> MEEIYAKFVSQKISKTRWRPLPPGSLQTAETFATGSWDNEENYISLWSIGDFGNLDSDGGFEGDHQLLCDIRHHGDVMDLQFFDQERIVAASSTGCV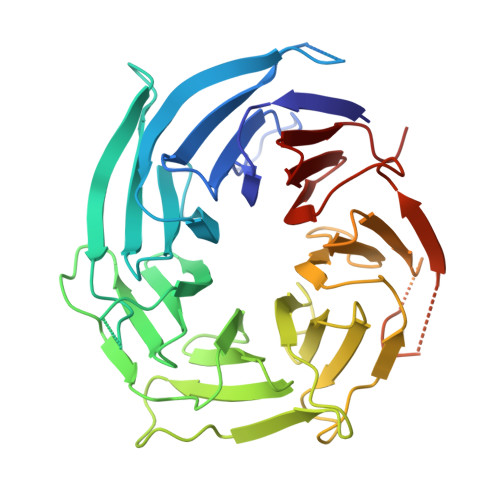TVFLHHPNNQTLSVNQQWTTAHYHTGPGSPSYSSAPCTGVVCNNPEIVTVGEDGRINLFRADHKEAVRTIDNADSSTLHAVTFLRTPEILTVNSIGQLKIWDFRQQGNEPSQILSLTGDRVPLHCVDRHPNQQHVVATGGQDGMLSIWDVRQGTMPVSLLKAHEAEMWEVHFHPSNPEHLFTCSEDGSLWHWDASTDVPEKSSLFHQGGRSSTFLSHSISNQANVHQSVISSWLSTDPAKDRIEITSLLPSRSLSVNTLDVLGPCLVCGTDAEAIYVTRHLFS> MPPKKQQEVVKVQWGRPGNNLKTGIVGMPNVGKSTFFRAITKSVLGNPANYPYATIDPEEAKVAVPDERFDWLCEAYKPKSRVPAFLTVFDIAGLTKGASTGVGLGNAFLSHVRAVDAIYQVVRAFDDAEIIHVEGDVDPIRDLSIIVDELLIKDAEFVEKHLEGLRKITSRGANTLEMKAKKEEQAIIEKVYQYLTETKQPIRKGDWSNREVEIINSLYLLTAKPVIYLVNMSERDFLRQKNKYLPKIKKWIDENS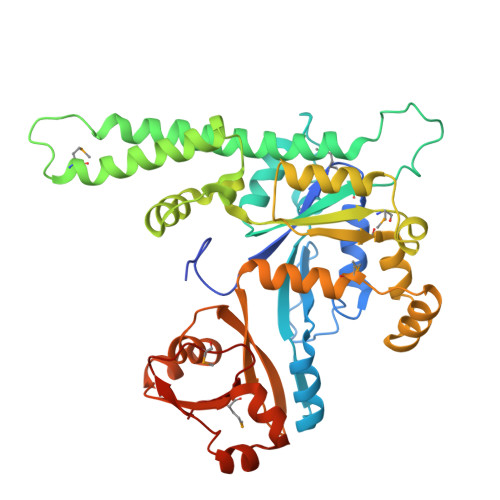PGDTLIPMSVAFEERLTNFTEEEAIEECKKLNTKSMLPKIIVTGYNALNLINYFTCGEDEVRSWTIRKGTKAPQAAGVIHTDFEKAFVVGEIMHYQDLFDYKTENACRAAGKYLTKGKEYVMESGDIAHWKAGKR> GMEQHQVWAYQTKTHSVTLNSVDIPALAADDILVQNQAIGINPVDWKFIKANPINWSNGHVPGVDGAGVIVKVGAKVDSKMLGRRVAYHTSLKRHGSFAEFTVLNTDRVMTLPDNLSFERAAALPCPLLTAWQAFEKIPLTKQREVLIVGFGAVNNLLTQMLNNAGYVVDLVSASLSQALAAKRGVRHLYREPSQ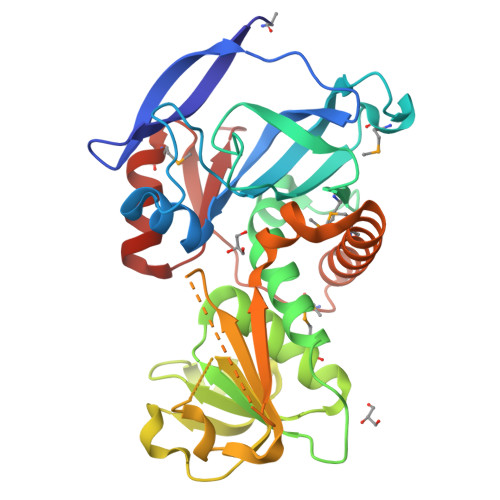VTQKYFAIFDAVNSQNAAALVPSLKANGHIICIQDRIPAPIDPAFTRTISYHEIALGALHDFGDRQDWQILMQQGEALLTLIAQGKMEIAAPDIFRFEQMIEALDHSEQTKLKTVLTLNE D-fructuronic 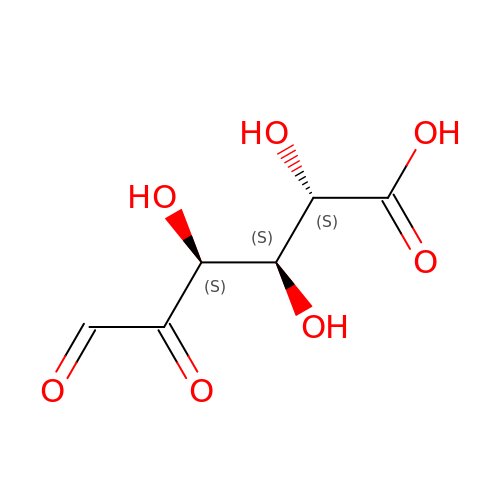acid | C6 H8 O7 | VLFFNIKCNGLGIG-WISUUJSJSA-N> XWTWNAYAFAAPS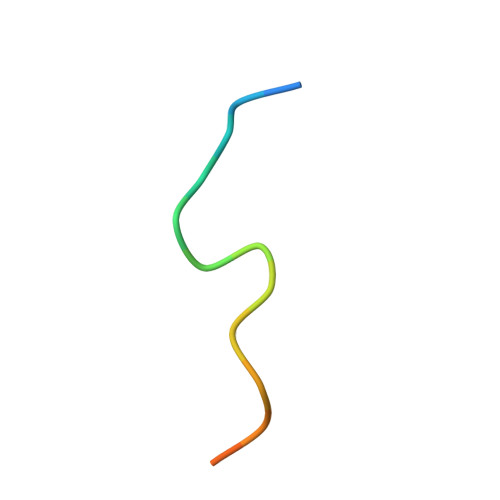GGGS> RPSWTVDSDSAKYSSFLDSLREEFGRGTPKVCNIPVTKKANNDKFVLVNLVLPFNRNTI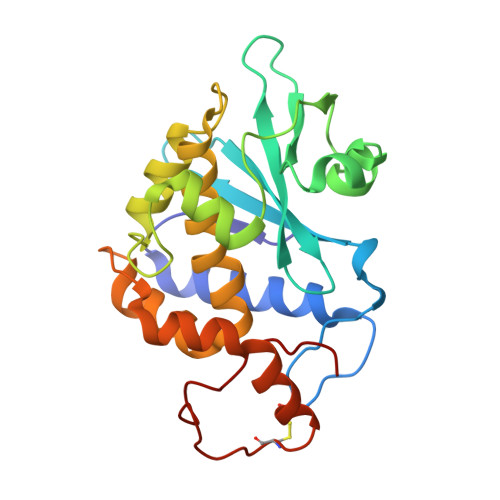TLAFRASDAYLVGFQDRDSKTNKLRANFFSDEYRALSGKYKSIFTDAEVLAPALPCASTYTDLQNKAGVSREKLSLGVSSLQTAFTAVYGKVFTGKNVAKFALISIQMVAEAARFKYIEDQVINRGMYSSFEAGARITLLENNWSKISEQYHKSCKLGGGQFTEEEMKLGLLLYN>[12x]MSIVTKSIVNADAEARYLSPGELDRIKAFVTGGAARLRIAETLTGSRETIVKQAGDRLFQKRPDIVSPGGNAYGEEMTATCLRDMDYYLRLVTYGVVSGDVTPIEEIGLVGVREMYRSLGTPIEAVAQSVREMKEVASGLMSSDDAAEASAYFDFVIGKMS;>[12x]MQDAITAVINSADVQGKYLDGAAMDKLKSYFASGELRVRAASVISANAATIVKEAVAKSLLYSDVTRPGGNMYTTRRYAACIRDLDYYLRYATYAMLAGDASILDERVLNGLKETYNSLGVPISSTVQAIQAIKEVTASLVGADAGKEMGVYLDYICSGLS;>MRMFRITACVPSQTRIRTQRELQNTYFTKLVPYDNWFREQQRIMKMGGKIVKVELATGRPGTNAGLA[2x];>[2x]MSVKASGGSSLARPQLYQTVPVSAISQAEQQDRFLEGSELNELTAYFQSGALRLEIAETLTQNADLIVSRAANRIFTGGSPLSYLEKPVERQPALVGASSDSRNGSVTYAESNGSGGLFGGLRSVFSSTGPIPPGFRPINIARYGPSNMQK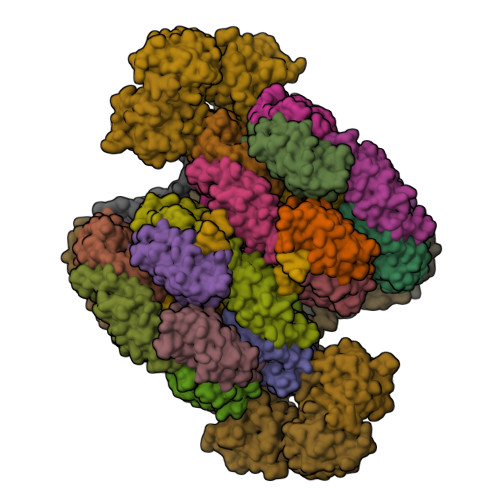SLRDMSWFLRYTTYAIVAGDPNIIVVNTRGLKEVIENACSIDATIVAIQEMRAASADYFRNNAQAKEIVLQYFDILLSEFKAPTPANKVRQGPSNDIQGLELPQSYFNAAAKRQKYAMKPGLSALEKNAVIKAAYRQIFERDITKAYSQSISYLESQVRNGDISMKEFVRRLAKSPLYRKQFFEPFINSRALELAFRHILGRGPSSREEVQKYFSIVSSGGLPALVDALVDSQEYADYFGEETVPYLRGLGVEAQECRNWGMQQDLFSYSAPFRKVPQFITTFAQYDRPLPDQHVYGSGNDPLEIQFGAIFPKETRNPSKRPAPFNKDTKRILIHRGPAVNNQVGNPSAVGEFPGSLGAKVFRLNGGLPGAKVGKNTGTSVKFGESSTQALIRAAYRQVFGRDLYEGQRLSVAEIQLENGDISVREFIKRLAKSELFLKLYWAPHYVCKAIEYMHRRLLGRPTYGRQEMNQYFDIASKQGFYAVVEAMIDSKEYSDAFGEDTVPYERYLTPGGLQMRSARVGSLREDIGQRVDKEVTPRFVELGQVSAIRTEPEIAYRSNQGVTRQRQQTKVFKLVSTYDKVAVKNAIRAAYRQVFERDLEPYIINSEFTALESKLSNNEINVKEFIEGLGTSELYMKEFYAPYPNTKVIEMGTKHFLGRAPLNQKEIQQYNQILASQGLKAFIGAMVNGMEYLQTFGEDTVPYRRFPTLPAANFPNTERLYNKLTKQDKELVVPSFTPVVKVGG;>[4x]MPFTIDSARGIFPNTLAADVVPATIARFSQLNAEDQLALIWFAYLEMGKTLTIAAPGAASMQLAENALKEIQAMGPLQQTQAMCDLANRADTPLCRTYASWSPNIKLGFWYRLGELMEQGFVAPIPAGYQLSANANAVLATIQGLESGQQITVLRNAVVDMGFTAGKDGKRIAEPVVPPQDTASRTKVSIEGVTNATVLNYMDNLNANDFDTLIELFTSDGALQPPFQRPIVGKENVLRFFREECQNLKLIPERGVTEPAEDGFTQIKVTGKVQTPWFGGNVGMNIAWRFLLNPEGKIFFVAIDLLASPKELLNFAR;>[4x]MALPLLNYAPKSQNVRVEGYEIGSEEKPVVFTTENILSSSDMDNLIEAAYRQIFFHAFKWDREKVLESQLRNGQITVRDFVRGLLLSNTFRNSFYEKNSNYRFVEHCVQKILGRDVYSEREKIAWSIVVATKGYQGLIDDLLNSDEYLNNFGYDTVPYQRRRNLPGREAGELPFNIKSPRYDAYHRRQLGFPQIVWQNEVRRFIPQEKKLTAGNPMNFLGMARSINPAANTIPKVSAQNINIEASVPRR>MEIHTYEKEFFDLLKRISHYSEAVALMHWDSRTGAPKNGSEDRAESIGQLSTDIFNIQTSDRMKELIDVLYERFDDLSEDTKKAVELAKKEYEENKKIPEAEYKEYVILCSKAETAWEEAKGKSDFSLFSPYLEQLIEFNKRFITYWGYQEHPYDALLDLFEPGVTVKVLDQLFAELKEAIIPLVKQVTASGNKPDTSFITKAFPKEKQKELSLYFLQELGYDFDGGRLDETVHPFATTLNRGDVRVTTRYDEKDFRTAIFGTIHECGHAIYEQNIDEALSGTNLSDGASMGIHESQSLFYENFIGRNKHFWTPYYKKIQEASPVQFKDISLDDFVRAINESKPSFIRVEADELTYPLHIIIRYEIEKAIFSNEVSVEDLPSLWNQKYQDYLGITPQTDAEGILQDVHWAGGDFGYFPSYALGYMYAAQLKQKMLEDLPEFDALLERGEFHPIKQWLTEKVHIHGKRKKPLDIIKDATGEELNVRYLIDYL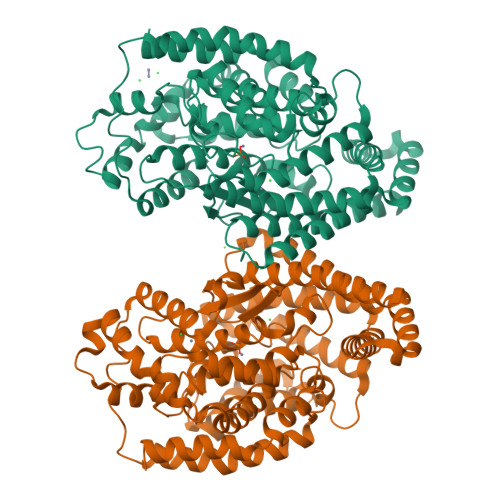SNKYSNLYLL[2x]> DPSLNNPVVIQATRLDASILPRNVFSKSYLLYVIAQGTDVGAIAGKANEAGQGAYDAQ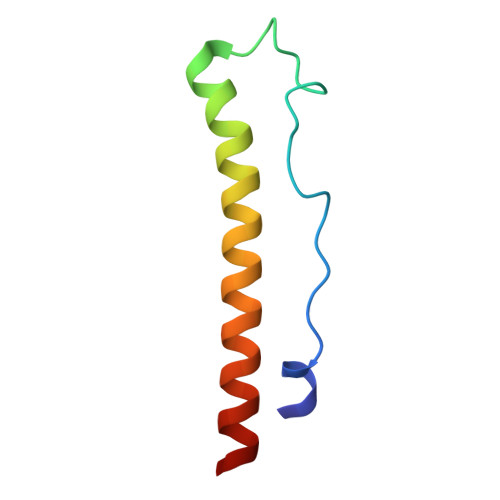VKND> VVGGEDAKPGQFPWQVVLNGKVDAFCGGSIVNEKWIVTAAHCVETGVKITVVAGEHNIEETEHTEQKRNVIRIIPHHNYNAAINKYNHDIALLELDEPLVLNSYVTPICIADKEYTNIFL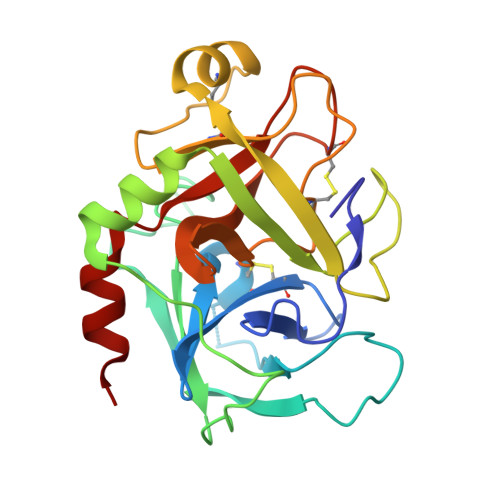KFGSGYVSGWGRVFHKGRSALVLQYLRVPLVDRATCLRSTKFTIYNNMFCAGFHEGGRDSCQGDSGGPHVTEVEGTSFLTGIISWGEECAMKGKYGIYTKVSRYVNWIKEKTKL>GGGGGGMSIRSLFGGLREKILGKNMKIVFPEGNDERVVRAAARLKFEGLLEPIILGQSEEVRNLLTKLGFADQDYTIINPNEYADFDKMKEAFVEVRKGKATLEDADKMLRDVNYFGVMLVKMGLADGMVSGAIHSTADTVRPALQIIKTKPGISRTSGVFLMNRENTSERYVFADCAINIDPTAQELAEIAVNTAETAKIFDIDPKIAMLSFSTKGSGKAPQVDKVREATEIATGLNPDLALDGELQFDAAFVPETAAIKAPDSAVAGQANTFVFPDLQSGNIGYKIAQRLGMFDAIGPILQGLNKP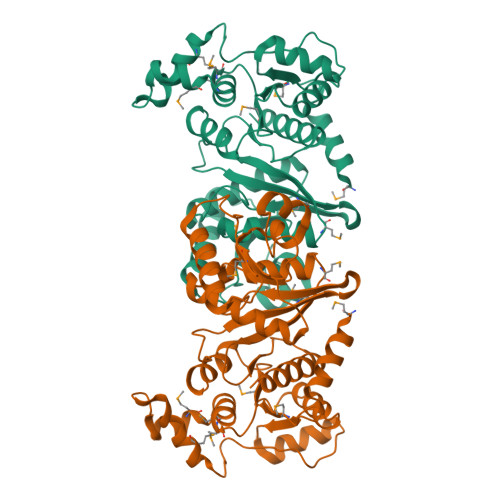VNDLSRGSSAEDIYKLAIITAAQAIESQG[2x]> PEKRVASSVFIT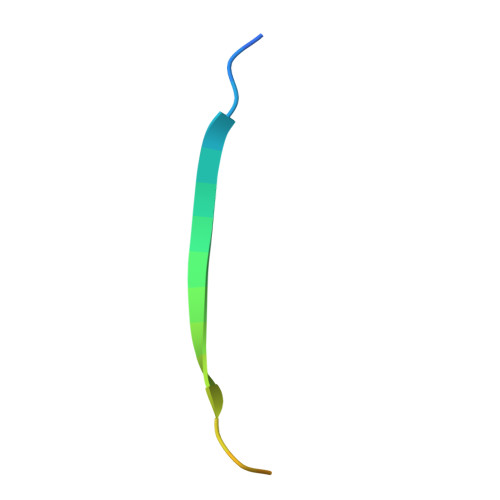LAPPRRDVAVAE> GPHMPGSGQIQLWQFLLELLSDSANASCITWEGTNGEFKMTDPDEVARRWGERKSKPNMNYDKLSRALRYYYDKNIMTKVHGKRYAYKFDFHGIAQALQPHPTE;> AELVRTDSPNFLCSVLPSHWRCNKTLPVAFKVVALGEVPDGTVVTVMAGNDENYSAELRNASAVMKNQVARFNDLRFVGRSGRGKSFTLTITVFTNPPQVATYHRAIKVTVDGPREPRRHRQKLDDSKPSLFSDRLSDLGRIPHPSMRVGVPPQNPRPSLNSAPSPFNPQGQ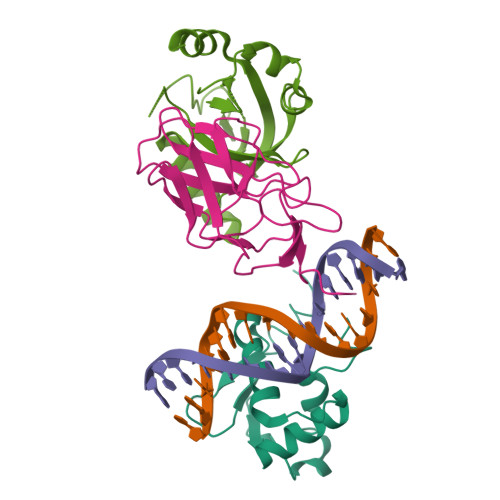SQITD;> MGSSHHHHHHSQDPMPRVVPDQRSKFENEEFFRKLSRECEIKYTGFRDRPHEERQARFQNACRDGRSEIAFVATGTNLSLQFFPASWQGEQRQTPSREYVDLEREAGKVYLKAPMILNGVCVIWKGWIDLQRLDGMGCLEFDEERAQQEDALAQQA> MKIVAIGAIPFSIPYTKPLRFASGEVHAAEHVLVRVHTDDGIVGVAEAPPRPFTYGET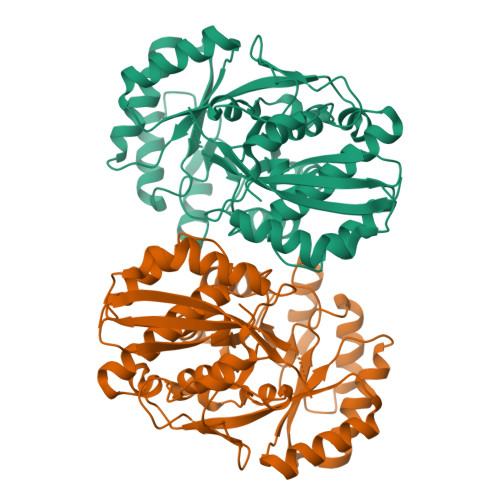QTGIVAVIEQYFAPALIGLTLTEREVAHTRMARTVGNPTAKAAIDMAMWDALGQSLRLSVSEMLGGYTDRMRVSHMLGFDDPVKMVAEAERIRETYGINTFKVKVGRRPVQLDTAVVRALRERFGDAIELYVDGNRGWSAAESLRAMREMADLDLLFAEELCPADDVLSRRRLVGQLDMPFIADESVPTPADVTREVLGGSATAISIKTARTGFTGSTRVHHLAEGLGLDMVMGNQIDGQIGTACTVSFGTAFERTSRHAGELSNFLDMSDDLLTVPLQISDGQLHRRPGPGLGIEIDPDKLAHYRTDN> GSAMGSSAADQQFYGQLQQELPQMVQQINSSDMQEQLAATVKFRQILSREHNPPIDIVIQSGVVPTLVNFMNENQPEMLQLEAAW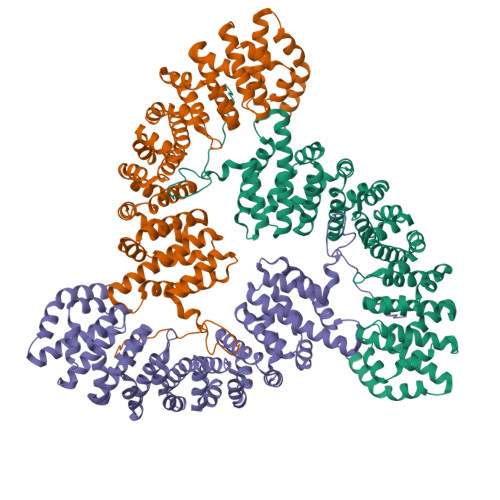ALTNIASGTSAQTQVVVDAGAVPLFIQLLYTGSVELQEQAIWALGNVAGDSTSYRDYVLQCSAMEPILSLFNSEKVTLIRTATWTLSNLCRGKKPQPDWSIVSKALPTLAKLIYSFDNETLIDACWAISYLSDGPAEAIQAVIDARIPKRLVELLSHQSTLVQTPALRAVGNIVTGNDLHTQVVINCGVLSALRNLLSSPKESIRKEACWTISNITAGNTEQIQAVVDANLIPPLIKLLETAEYKIKKEACWAISNASSGGLQRPEIIRYMVSQGCIKPLCDLLEIADNRIIEVTLDALENILKMGETDKEARGLAINENADLIEKAGGMEKIFNCQQNENDRIYEKAYKIIETYFGEELVPRGSEVNGKRVSKTSTGKRKFHKKSKTG>GPLGSMANRDDIDASAVMAAYLAREYAEAV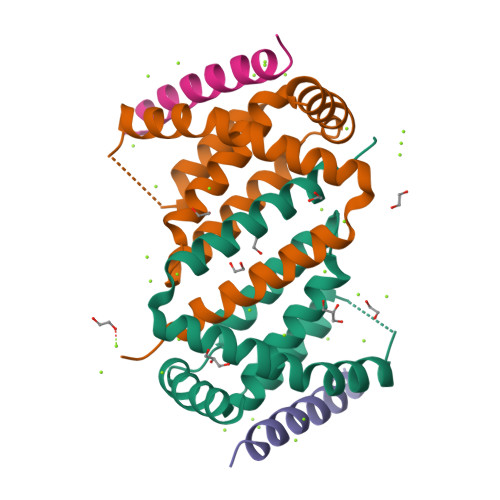EEQLTPRERDALEALRVSGEEVRSPLLQELSNAGEHRANPENSHIPAALVSALLEAPTSPGRMVTAVELCAQMGRLWTRGRQLVDFMRLVYVLLDRLPPTADEDLGAWLQAVARVHGT[2x];>[2x]VPQDASTKKLSECLKRIGDELDSNMELQ> GMFLLQGAQMLQMLEKSLRKSLPMSLKVYGTVMHMNHGNPFNLKALVDKWPDFQTVVIRPQEQDMKDDLDHYTNTYHVYSEDLKNCQEFLDLPEVINWKQHLQIQSTQSSLNEVIQNLAATKSFKVKRSKNILYMASETIKELTPSLLDVKNLPVGDGKPKAIDPEMFKLSSVDPSHAAVVNRFWLFGGNERSLRFIERCIQSFPNFCLLGPEGTPVSWSLMDQTGEMRMAGTLPEYRAQGLVTHAIYQQAQCLLKRGFPVYSHVDPKNQIMQKMSQSL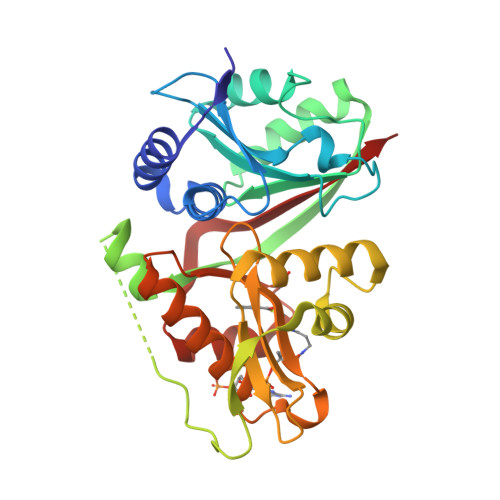NHVPMPSDWNQWNCEPL The NanH sialidase of Tannerella forsythia, one of the bacteria associated with severe periodontal disease plays a role in virulence. The C-terminal catalytic domain is preceded by a 160 amino acid N-terminal domain that is a CBM that our laboratory discovered is capable of binding various sialoglycans and non-sialylated derivatives but has no catalytic activity itself. The NanH catalytic domain (residues 197–552) folds into a characteristic 6-bladed β-propeller catalytic domain, with each blade being composed of 3–4 antiparallel β-strands.

We also use non-catalytic (D237A) variant to characterise molecular interactions while in complex with the natural substrates 3- and 6-siallylactose. Using this mutant we produced crystals and determined structures for the NanH-D237A-apo protein (1.7 Å) and complexes with 3-SL (2.06 Å) and 6-SL (1.90 Å). As might be expected, the terminal sialic acid of 3-SL and 6-SL are positioned in the active site of NanH-D237A with their carboxyl-groups (C1) co-ordinated by a hydrogen bonding network with the arginine triad residues (R423, R487 and R212) and the N-acetyl group hydrogen bonds with D280 in a similar manner to that seen in the NanH-oseltamivir model. The pyranose ring sits in a distorted boat conformation, while as a result of the D237A mutation, the C4-OH group makes contact with R231. Of note here, when the 3-SL and 6-SL structural models are overlaid, the sialic acid portion of 6-SL occupies a near identical space to that of 3-SL with no substantial differences (≥0.1 Å) between the hydrogen bond lengths connecting the 3-SL and 6-SL terminal sialic acids to the conserved catalytic residues. Perhaps unsurprisingly the glycosidic linkage between C2 of sialic acid and the underlying galactose is in a near identical position in 3D space for both the 3-SL and 6-SL models, a phenomenon also seen in other proteins — such as Influenza A (HA) — the only other sialidase structures with these substrates in the active site. The galactose of the 3-SL complex is perpendicular to the sialic acid residue and pointing out of the active site whilst in contrast, the angle made by the galactose to the sialic acid in the 6-SL structure is different and directs the galactose into the central cleft of the enzyme dimer. In both cases no hydrogen bonding network could be seen between galactose and the protein backbone, indicating it may exist in various orientations. Of note, there is no displacement of W308 in the 3-SL or 6-SL models in contrast with the NanH-oseltamivir model.

>DSVYVQNPQIPILVDRTDNVLFRIRIPDATKGDVLNRLTIRFGNEDKLSEVKAVRLFYAGTEAATKGRSRFAPVTYVSSHNIRNTRSANPSYSIRQDEVTTVANTLTLKTRQPMVKGINYFWVSVEMDRNTSLLSKLTSTVTEVVINDKPAVIAGEQAAVRRMGIGVRHAGDDGSASFRIPGLVTTNKGTLLGVYDVRYNNSVALQEHIDVGLSRSTDKGQTWEPMRIAMSFGETDGLPSGQNGVGDPSILVDERTNTVWVVAAWTHGMGNARAWTNSMPGMTPDETAQLMMVKSTDDGRTWSESTNITSQVKDPSWCFLLQGPGRGITMRDGTLVFPIQFIDSLRVPHAGIMYSKDRGETWHIHQPARTNTTEAQVAEVEPGVLMLNMRDNRGGSRAVSITRDLGKSWTEHSSNRSALPESICMASLISVKAKDNIIGKDLLLFSNPNTTEGRHHITIKASLDGGVTWLPAHQVLLDEEDGWGYSCLSMIDRETVGIFYESSVAHMTFQAVKIKDLIR[2x]>SNAMAVLLSGVPVLAALDVSTTQKFWIEVLGFTEEFLTEDFGGVSRDGVELFICSVEDQVVPDNTQAWLRVRDIDAL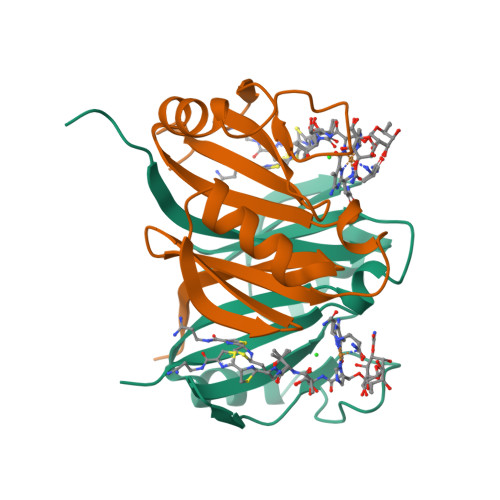HAEWSARVSSDYADASHPAMTAIREVPWGREFGLRDPAGNLVHFSELSEAAETTRTVR[2x]>[2x]MHHHHHHSSGRENLYFQGTGQDALVLGFDWGKFLKDHSYKAA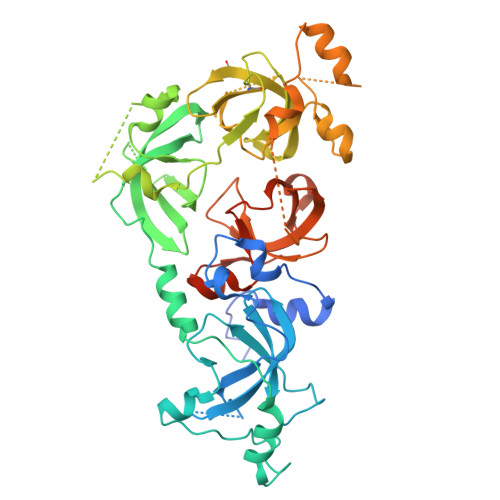PVSCFKHVPLYDQWEDVMKGMKVEVLNSDAVLPSRVYWIASVIQTAGYRVLLRYEGFENDASHDFWCNLGTVDVHPIGWCAINSKILVPPRTIHAKFTDWKGYLMKRLVGSRTLPVDFHIKMVESMKYPFRQGMRLEVVDKSQVSRTRMAVVDTVIGGRLRLLYEDGDSDDDFWCHMWSPLIHPVGWSRRVGHGIKMSERRSDMAHHPTFRKIYCDAVPYLFKKVRAVYTEGGWFEEGMKLEAIDPLNLGNICVATVCKVLLDGYLMICVDGGPSTDGLDWFCYHASSHAIFPATFCQKNDIELTPPKGYEAQTFNWENYLEKTKSKAAPSRLFNMDCPNHGFKVGMKLEAVDLMEPRLICVATVKRVVHRLLSIHFDGWDSEYDQWVDCESPDIYPVGWCELTGYQLQPPVAAEPATPLKAKEATKKKKKQ>GNPIVVVHGGGAGPISKDRKERVHQGMVRAATVGYGILREGGSAVDAVEGAVVALEDDPEFNAGCGSVLNTNGEVEMDASIMDGKDLSAGAVSAVQCIANPIKLARLVMEKTPHCFLTDQGAAQFAAAMGVPEIPGEKLVTERNKKRLE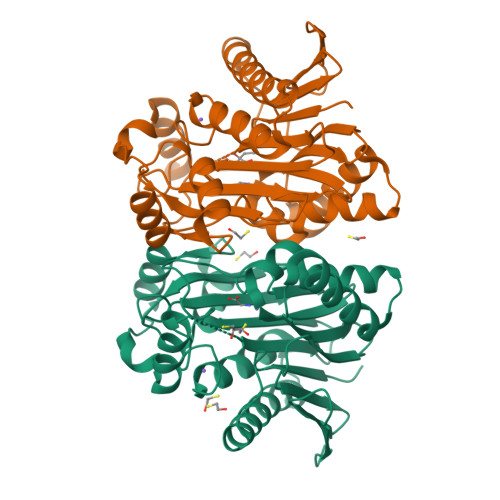KEKHEKGAQKTDCQKNLGHHHHHHMTVGAVALDCKGNVAYATSTGGIVNKMVGRVGDSPCLGAGGYADNDIGAVSTTGHGESILKVNLARLTLFHIEQGKTVEEAADLSLGYMKSRVKGLGGLIVVSKTGDWVAKWTSTSMPWAAAKDGKLHFGIDPDDTTITDLPGAGSGAGSGAGG[4x]> MPRRSARKAQSAIASPADTNVVPAKDAPTTNSPPSTTSPNQAAADANQQQAGIVSSQSGPNAVGDSAPSSSVNNDGDIITRPTSDSIAAVANATKPAAVVSDPQSMKVTPIVNPSSYVCNVCNARFSTMSALSEHLRSDHRDDASTLLATPMINNAIRSFLTAWDDIRILSPDVSSKSLSAYLDSAVANGPELIIEDTGLCTSFMLLDNIPSAHLTKELIGFTWFMQMYQMTPPLPEGAVNRIVCMTNWASLGDEGRGLEVRLPPPTDSSVHAYKTVLSRGYIDNAQFNPLALRSNVLLMLLQFTLSNLKINKSSTFTSDVTTITSGRMIRAFEGRPELLALAYPGRAVLPTQTKNAQFLSTAIADRIGRLDRANLIGGEVSAMVECMELCDALTLHIRETYIMLLRSMHQDPTQIVQIVNECANNLLNSTIPISLRPTILCPWFASSEDLRLQQVMHLVNISSNTAAALPLVEALSTLLRSVTPLVLDPTVLTNAITTISESTTQTISPISEILRLLQPMGNDYAAFWKCIASWAYNGLVTTVLSEDAFPDSSQSITHLPSMWKCLFLTLAGPMTSDPHSPVKVFMALANLLAQPEPIAIGVPGMHQTTPASQFSHPGVWPPGFLNPQLINPQQAPLLRAFAEHIRANWPQPSEFGYGSTLQGSANLFIPSNRMVYPWPNQPLPRLTVAPTYDSAMSNWISTTIAFFIRVVNSVNMTATVNDLTRRTMTGVMTAMRQVKTMTPFYIQHMCPTELSVLASVTVTPPFQVPFTRLVQNDVITNVLVARVDPAQRGDAAVDIRATHATFAAALPVDPAAIVVAMLCGQTETNLIPSHHYGKAFAPLFASNAMFTRNQRAVITREAFVCARSAVAQCQDAGFLVPRPLDALRQFDVTSAAAAEIMHAVNDAFKTAFDLDGALLDGLALYGDPRIADLSAAYLQYGGNVVREHVPPGPSHIHRALQQVESTFMAEMNLFNVARGNLYLVQTATNGNWSPMAPVAAPPFVRGGPNVRVVGRFGTIVPRPNGLEPQLIDDGNVPRDIAGDWVYPSDVLQVSVAVFRDYVWPMVKAGRTRVLVELGHYVYTLHYYDPQISLDEAPI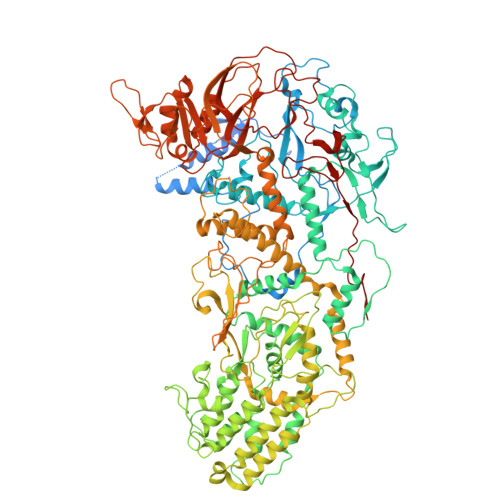LEEWLSKINPAGIPPVPFCIPIPQVYPCITARRVHYAFTSENNNDSLFSTNAASIDTAFGENAAVSPLRWPGLVDPNYRVGTNDLPNRITLYNSLYRYNFTYPTLDGIMYVRSAT> MESITVTELKEKILDANPVNIVDVRTDQETAMGIIPGAETIPMNSIPDNLNYFNDNETYYIICKAGGRSAQVVQYLEQNGV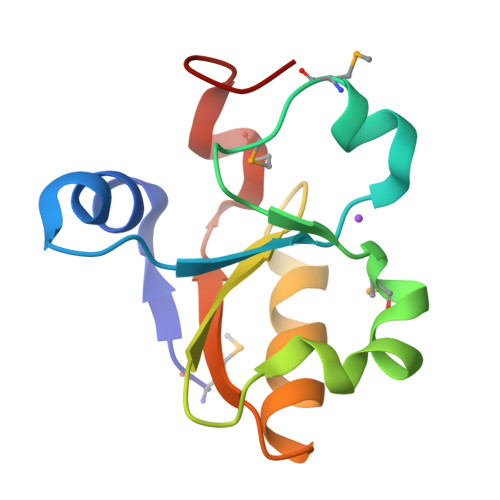NAVNVEGGMDEFGDEGLEH> MNHKVHHHHHHIEGRSMACTIQKAEALDGAHLMQILWYDEEESLYPAVWLRDNCPCSDCYLDSAKARKLLVEALDVNIGIKGLIFDRKKVYITWPDEHYSEFQADWLKKRCFSKQARAKLQRELFFPECQYWGSELQLPTLDFEDVLRYDEHAYKWLSTLKKVGIVRLTGASDKPGEVSKLGKRMGFLYLTFYGHTWQVQDKIDANNVAYTTGKLSFHTDYPALHHPPGVQLLHCIKQTVTGGDSEIVDGFNVCQKLKKNNPQAFQILSSTFVDFTDIGVDYCDFSVQSKHKIIELDDKGQVVRINFNNATRDTIFDVPVERVQPFYA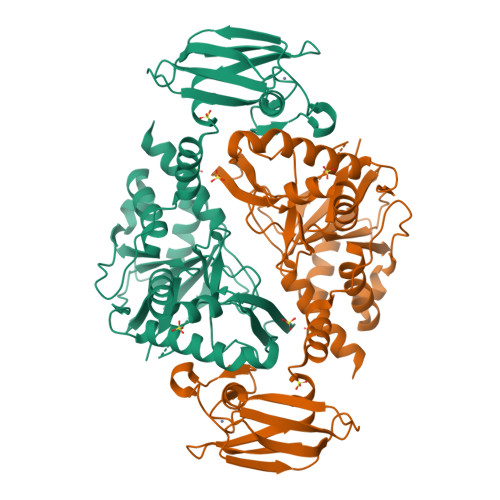ALKEFVDLMNSKESKFTFKMNPGDVITFDNWRLLHGRRSYEAGTEISRHLEGAYADWDVVMSRLRILRQRVENGN> MSSNVGTIANA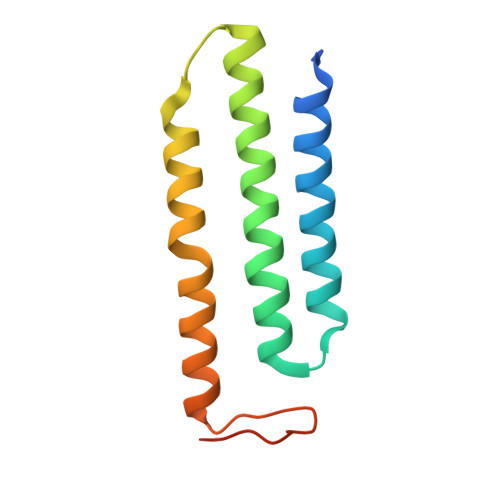LVVVLILLGAVLTLLSAVGAIRLPDVYTRSHAISKSTTLGIMCILLGAFLHFFIENNHFNSRLLLGIVFIFMTSPVAAHLISRAAYYANVERWEGTVRDDLKQKAGGK> MVDPLMTNAPPEPCDLLIEAGYVVPIEPHAVVLEDHAVAVSNGVIVAVLPTADARVRFAPARTVSRPDAALMPGLVNAHTHNPMTLLRGVADDLPLMVWLQQHIWPVEAAVIGPEFVADGTTLAIAEMLRGGTTCVNENYFFADVQAAVYKQHGFRALVGAVIIDFPTAWASSDDEYFARAGELHDQWRDDPLISTAFAPHAPYTVNDANFERVRMLADQLDMPVHLHTHETAQEVADSVAQYGQRPLARLDRLGLVNDRLIAVHMTQLTEAEIHLCAERGVSVVHCPESNLKLASGFCPACALQRASVNLAIGTDGCASNNDLDMFSENRTAAILAKAVANDATALDAATTLRAATLGGARALGFGDRIGSIEVGKQADLVCVDLSA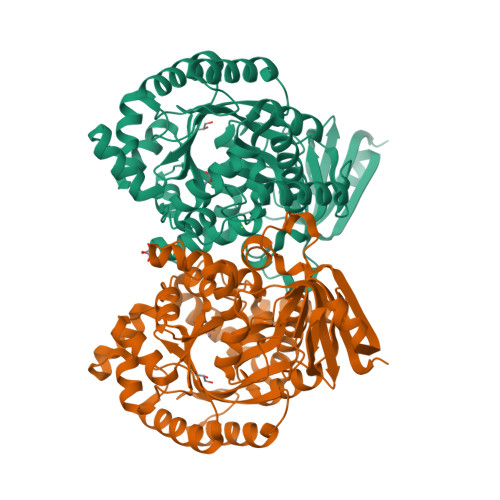LETQPLHHVLSQLIYAAGRHQVTDVWIAGKPKLVQRELIDMDTAALVANARQWRDRIRTVRAAENLYFQSHHHHHHWSHPQFEK>[2x]PYAESYIDTVQDRMKQRDRESKLTGKPINMQEQIIDGWFLARFWIFKDQNNNHQTNRFISWFKDNLASSKGYDSIAEQMGLKIEALNDMDVTNIDYTSKTGDTIYNGISELTNYTGTTQKMKTDSFQRDYTKSESTSVTNGLQLGFKVA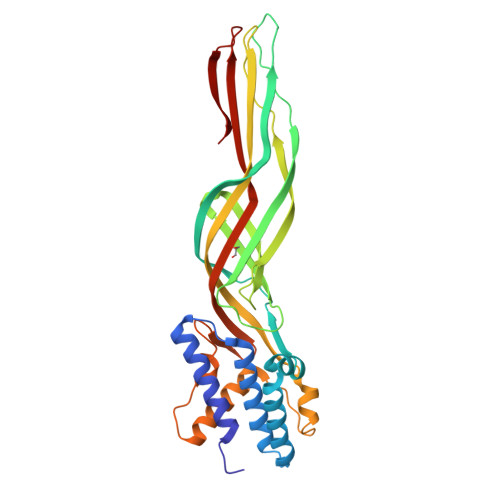AKGVVALAGADFETSVTYNLSSTTTETNTISDKFTVPSQEVTLSPGHKAVVKHDLRKMVYFGTQDLKGDLKVSFNDKEIVQKFIYPNYRSIDLSDIRKTMIEIDKWNHVNTIDFYQLVGVKNHIKNGDTLYIDTPAEFTFNGANPYYRATFTEYDENGNPVQTKILSG>[2x]MAEPATSGPYQWRSVAIGGGGFVTGVLFHPAERGLAYARTDVGGAYRWDAQAQQWTALTDWLGADDWNLMGIDAFAVDPADADALYLAAGTYMHERAGNAAVLRSFNRGRTFERADLPFKLGGNQLGRANGERLAVDPHDGRVLLLGSRDAGLWRSDDRGAHWAKVASFPDAALAGATARNHVGREQAVGIAFVVFDAASGNTGTPTPRIYVGVSTEQTSLYVSEDAGRSWAPVAGQPRGLRPSHMAGGSDGHWYLSYGDQPGPDLMAGGA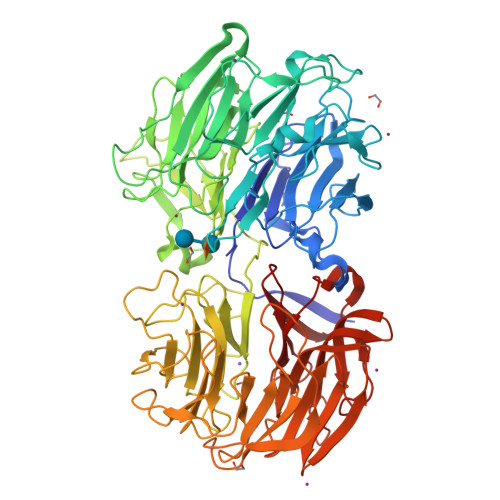LWKFTPAQGRWREISPIPQPASGDGFGWGAVAVDPQQPQVLLASTFRRRTPRDELYRSVDGGKHWAPLLADAVFDHSAAPWTAHATPHWMGALAIDPFDGNHALFVTGYGIWASRNLQDFAAPQRPLQWWFQDRGLEETVPLDLLSPMAGAHLLSALGDIDGFRHDELDRAQLQYAGPRLTNGESIDAAGQAPQWVVRSGTVRDRRNNEIRALYSRDGGKQWTAFASEPPAGQGAGSIAIGADAAQVVWAPERGGNWRTSDFGAQWQRVDGLPDTAVVMADRVDARRWYAVDVASGQLYESTDAARSFRATGVQVGSPARDERTRPQLRPDPWRAGVVYLASPGKGVMRWQDGTLQVLSQPDEARSLGIGKALRAGAPPALYLAGRVQGVDGVFRSDDGGVQWQRINDDAHRFGRPYSVTGDPRIAGRVYFATGGRGIFYGDPR The nef genes of human and simian immunodeficiency viruses (HIV-1, HIV-2, and SIV) encode accessory proteins of 27–35 kDa critical for viral pathogenesis. At the molecular level, Nef enhances viral infectivity and replication by stimulating multiple host cell signal transduction pathways. Nef also hijacks endocytic trafficking pathways to induce downregulation of viral receptors, including CD4 and chemokine receptors, and prevent cell-surface display of MHC-I in complex with HIV-1 antigens. The folded core domain exhibits the highest degree of sequence and structural conservation among Nef proteins.

The Nef protein used in this study is derived from the HIV-1 B-clade isolate SF2, and consists of residues 51–205 (numbering is based on the crystal structure of Nef NL4-3). The crystal structure of Nef (51–205) was determined at 3.2 Å, with six Nef molecules forming three identical homodimers in the asymmetric unit. The core domain consists of two anti-parallel α-helices (αA and αB), four central anti-parallel β-strands and a short C-terminal helix (αC). Notably, we observed one additional α-helix formed by residues 54–66 (designated helix α0), which is connected to the PXXP motif by residues 67-GFPVR-71. Helix α0 packs against helix αB and is connected to helix αA by a long loop containing the PXXP motif, so as to form an α0-αB-αA helix array. The total buried surface area between the two Nef monomers is about 2000 Å2, with helices α0, αA and αB from each Nef monomer involved in dimerization. Nef (51–205) helix B residues I109, L112, W113, H116, and the methyl group of T117 from both Nef monomers interact to create a hydrophobic pocket. The hydrophobic tail of βOG inserts into the hydrophobic pocket formed by the side chains of I109, L112, W113 and H116. In the Nef (51–205) dimer, the presence of βOG stabilizes a fairly compact and symmetrical dimer, with tight nearly parallel juxtaposition of the αB helices around the βOG molecule. However, when the experiment was repeated in the presence of the same concentration of βOG used for the crystallization studies (0.1%), the Nef peak shifted to a lower retention volume, consistent with dimer formation.

>[6x]ADCAWLEAQEEEEVGFPVRPQVPLRPMTYKAALDISHFLKEKGGLEGLIWSQRRQEILDLWIYHTQGYFPDWQNYTPGPGIRYPLTFGWCFKLVPVEPEKVEEANEGENNSLLHPMSLHGMEDAEKEVLVWRFDSKLAFHHMARELHPEYY Sliding clamps are ring-shaped protein complexes that are integral to the DNA replication machinery of all life. Sliding clamps are opened and installed onto DNA by clamp loader AAA+ ATPase complexes. The clamp loader of eukaryotes Replication Factor C (RFC) installs the sliding clamp Proliferating Cell Nuclear Antigen (PCNA) in a coordinated and stepwise fashion. In contrast to typical AAA+ ATPases, clamp loaders are heteropentameric with the five different subunits called A–E.

To our knowledge, these are the first high-resolution structures of a clamp loader bound to an open clamp prior to DNA binding. Both reconstructions are highly similar (overall Cα RMSD is 0.74 Å, map to map correlation coefficient is ~0.85) and we refer to these structures as Open1 and Open2. PCNA forms a right-handed spiral with a ~20 Å opening that is wide enough for dsDNA to enter. PCNA opens at the A-gate of RFC, disrupting the interaction between the first and third subunits of the PCNA ring (termed PCNA-I and PCNA-III, hereafter). The open PCNA ring is directly held by all five subunits of RFC, burying ~3800 Å2 of surface area, an approximate ~1860 Å2 increase over that of the Autoinhibited states. The AAA+ modules of RFC adopt a right-handed spiral whose periodicity matches that of the six contact sites on PCNA. In order to rupture the PCNA ring, the AAA+ spiral of RFC widens, opening the A-gate. The RFC-E subunit uses its E-plug to bind PCNA, which pulls the A′ domain and E-plug up to 45 Å away from the AAA+ module. This reveals a large opening of the A-gate (at its most narrow, the A-gate is approximately 20 Å wide). p/t-DNA can therefore directly enter the open RFC:PCNA complex. The Open1 and 2 states represent the stable intermediate state in which PCNA is opened but DNA has yet to bind.

> MVNISDFFGKNKKSVRSSTSRPTRQVGSSKPEVIDLDTESDQESTNKTPKKMPVSNVIDVSETPEGEKKLPLPAKRKASSPTVKPASSKKTKPSSKSSDSASNITAQDVLDKIPSLDLSNVHVKENAKFDFKSANSNADPDEIVSEIGSFPEGKPNCLLGLTIVFTGVLPTLERGASEALAKRYGARVTKSISSKTSVVVLGDEAGPKKLEKIKQLKIKAIDEEGFKQLIAGMPAEGGDGEAAEKARRKLEEQHNIATKEAELLVKKEEERSKKLAATRVSGGHLERDNVVREEDKLWTVKYAPTNLQQVCGNKGSVMKLKNWLANWENSKKNSFKHAGKDGSGVFRAAMLYGPPGIGKTTAAHLVAQELGYDILEQNASDVRSKTLLNAGVKNALDNMSVVGYFKHNEEAQNLNGKHFVIIMDEVDGMSGGDRGGVGQLAQFCRKTSTPLILICNERNLPKMRPFDRVCLDIQFRRPDANSIKSRLMTIAIREKFKLDPNVIDRLIQTTRGDIRQVINLLSTISTTTKTINHENINEISKAWEKNIALKPFDIAHKMLDGQIYSDIGSRNFTLNDKIALYFDDFDFTPLMIQENYLSTRPSVLKPGQSHLEAVAEAANCISLGDIVEKKIRSSEQLWSLLPLHAVLSSVYPASKVAGHMAGRINFTAWLGQNSKSAKYYRLLQEIHYHTRLGTSTDKIGLRLDYLPTFRKRLLDPFLKQGADAISSVIEVMDDYYLTKEDWDSIMEFFVGPDVTTAIIKKIPATVKSGFTRKYNSMTHPVAIYRTGSTIGGGGVGTSTSTPDFEDVVDADDNPVPADDEETQDSSTDLKKDKLIKQKAKPTKRKTATSKPGGSKKRKTKA;> MSKTLSLQLPWVEKYRPQVLSDIVGNKETIDRLQQIAKDGNMPHMIISGMPGIGKTTSVHCLAHELLGRSYADGVLELNASDDRGIDVVRNQIKHFAQKKLHLPPGKHKIVILDEADSMTAGAQQALRRTMELYSNSTRFAFACNQSNKIIEPLQSRCAILRYSKLSDEDVLKRLLQIIKLEDVKYTNDGLEAIIFTAEGDMRQAINNLQSTVAGHGLVNADNVFKIVDSPHPLIVKKMLLASNLEDSIQILRTDLWKKGYSSIDIVTTSFRVTKNLAQVKESVRLEMIKEIGLTHMRILEGVGTYLQLASMLAKIHKLNNKA;> MSTSTEKRSKENLPWVEKYRPETLDEVYGQNEVITTVRKFVDEGKLPHLLFYGPPGTGKTSTIVALAREIYGKNYSNMVLELNASDDRGIDVVRNQIKDFASTRQIFSKGFKLIILDEADAMTNAAQNALRRVIERYTKNTRFCVLANYAHKLTPALLSRCTRFRFQPLPQEAIERRIANVLVHEKLKLSPNAEKALIELSNGDMRRVLNVLQSCKATLDNPDEDEISDDVIYECCGAPRPSDLKAVLKSILEDDWGTAHYTLNKVRSAKGLALIDLIEGIVKILEDYELQNEETRVHLLTKLADIEYSISKGGNDQIQGSAVIGAIKASFENETVKANV;> MFEGFGPNKKRKISKLAAEQSLAQQPWVEKYRPKNLDEVTAQDHAVTVLKKTLKSANLPHMLFYGPPGTGKTSTILALTKELYGPDLMKSRILELNASDERGISIVREKVKNFARLTVSKPSKHDLENYPCPPYKIIILDEADSMTADAQSALRRTMETYSGVTRFCLICNYVTRIIDPLASRCSKFRFKALDASNAIDRLRFISEQENVKCDDGVLERILDISAGDLRRGITLLQSASKGAQYLGDGKNITSTQVEELAGVVPHDILIEIVEKVKSGDFDEIKKYVNTFMKSGWSAASVVNQLHEYYITNDNFDTNFKNQISWLLFTTDSRLNNGTNEHIQLLNLLVKISQL;> MSLWVDKYRPKSLNALSHNEELTNFLKSLSDQPRDLPHLLLYGPNGTGKKTRCMALLESIFGPGVYRLKIDVRQFVTASNRKLELNVVSSPYHLEITPSDMGNNDRIVIQELLKEVAQMEQVDFQDSKDGLAHRYKCVIINEANSLTKDAQAALRRTMEKYSKNIRLIMVCDSMSPIIAPIKSRCLLIRCPAPSDSEISTILSDVVTNERIQLETKDILKRIAQASNGNLRVSLLMLESMALNNELALKSSSPIIKPDWIIVIHKLTRKIVKERSVNSLIECRAVLYDLLAHCIPANIILKELTFSLLDVETLNTTNKSSIIEYSSVFDERLSLGNKAIFHLEGFIAKVMCCLD;>PHMASMLEAKFEEASLFKRIIDGFKDCVQLVNFQCKEDGIIAQAVDDSRVLLVSLEIGVEAFQEYRCDHPVTLGMDLTSLSKILRCGNNTDTLTLIADNTPDSIILLFEDTKKDRIAEYSLKLMDIDADFLKIEELQYDSTLSLPSSEFSKIVRDLSQLSDSINIMITKETIKFVADGDIGSGSVIIKPFVDMEHPETSIKLEMDQPVDLTFGAKYLLDIIKGSSLSDRVGIRLSSEAPALFQFDLKSGFLQFFLAPKFNDEE[3x]>CGCAAATTTGCG[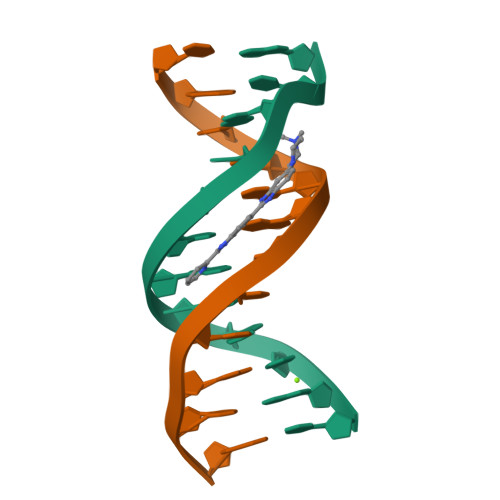2x]> MFRWLFLYWYNSTDTPSAIAKVNLWSYINLRLFKARL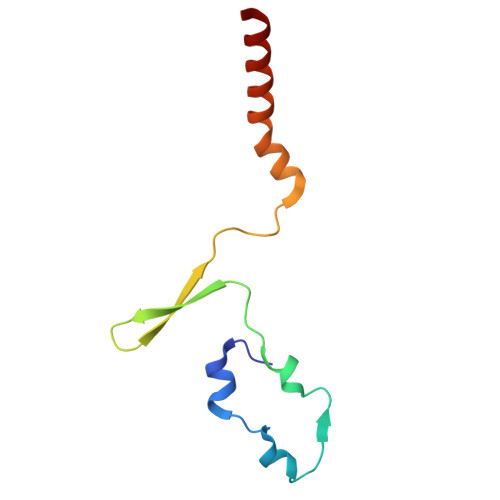SSSIAYYILGLNNLELKKLKIFYKNTYFDYIYLKSIPCLFLIIFFTNLYLFL>GITGTWYNQLGSTFIVTAGADGALTGTYESAVGNAESRYVLTGRYDSAPATDGSGTALGWTVAWKNNYRNAHSAT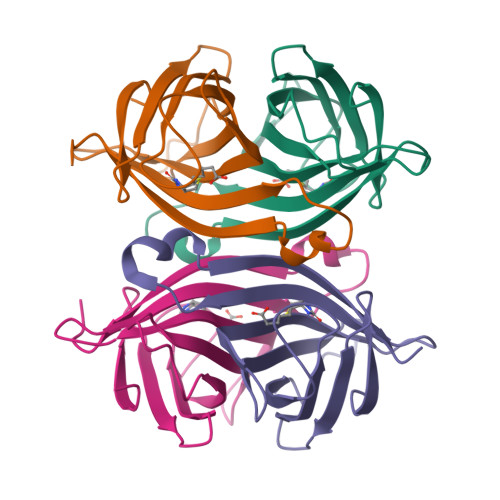TWSGQYVGGAEARINTQWLLTSGTTEANAWKSTLVGHNTFTKVKP[4x]>GGCGCC[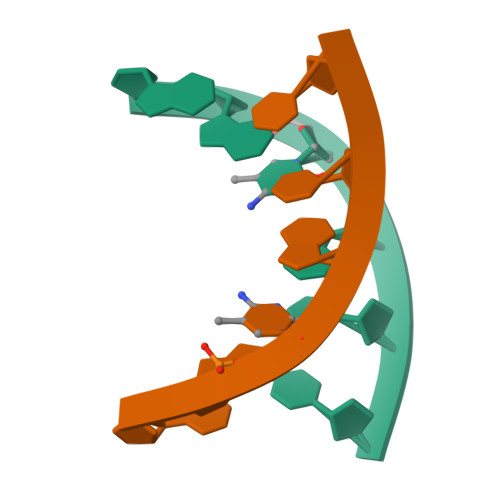8x]> MSALYFQNLPSRPANKENYTRLLLKHINPNNKYAINPSLPLP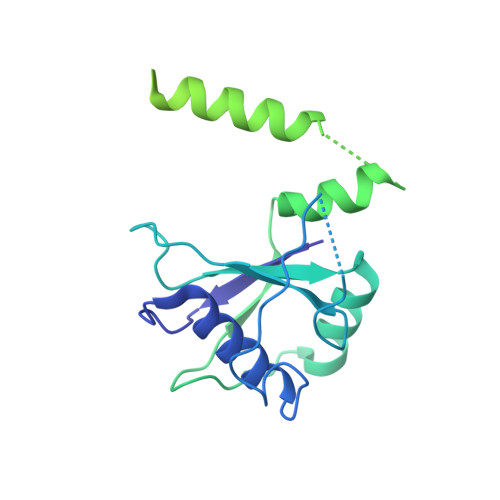HNKLQISSQPLMLLDDQMGLLEVSISRSSKMTNQAFLTFVTQEEADRFLEKYTTTALKVQGRKVRMGKARTNSLLGLSIEMQKKKGNDETYNLDIKKVLKARKLKRKLRSDDICAKKFRLKRQIRRLKHKLRSRKVEEAEIDRIVKEFETRRLENMKSQQENLKQSQKPLKRAKVSNTMENPPNKVLLIQNLPSGTTEQLLSQILGNEALVEIRLVSVRNLAFVEYETVADATKIKNQLGSTYKLQNNDVTIGFAK> MSNSAIPLNVVAVQEPRLELNNERTWVVVKGGQQVTYYPFPSTSFSSNQFNFICNPPSAQTVLDRLVFIQVPYDITFTANPSHAGITENLLQPGRDAFRAFPISSITNTLNATINGFPVNIELAQIIHALSRYHTPLKVKNGWMSMQPSFEDNYQSYRDADGANNNPLGVFTSAAGLSELPRGSYTMNVVTNTTTTARITGVLYEQVFLPPFLWDGEQAGGLANLTSLTFNWVLNNNLARIWSHSDITNDVSGNSTIGSMNISFQQPSMYLGFVTPRLNIPIPPRITYPYFKLSRYTTQFQNTLAPNASSTFKSNVVQLDSIPRKLYLFVKQSDNVIYQNLNNQITTPDVFLQINNLNLTWNNQQGILSGASSQNLYDFSVQNGYNKTWSEFNGVTQQFNGVSGQPTKVIGLEGGIVCLELGKDVGLRDDEAEGVIGNFNLQVQMTVTNTNQYVTVTPDMYIVAVYDGTLVISNTSAMASIGVASKEEVLNAR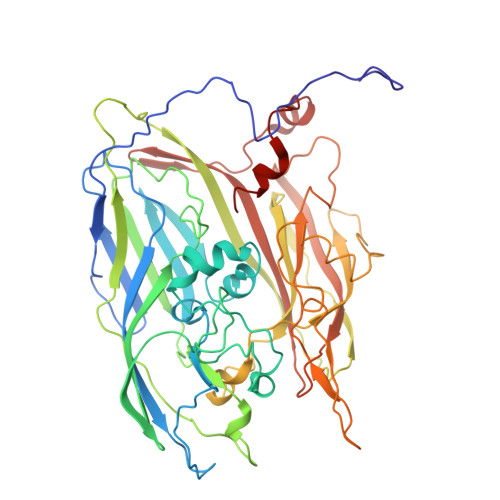ITHGVSYNELQRIYG>[2x]GPLGSMHNVLIVGASRGIGLGLADAFLQRGAQVFAVARRPQGSPGLQALAERAGERLQAVTGDLNQHDCA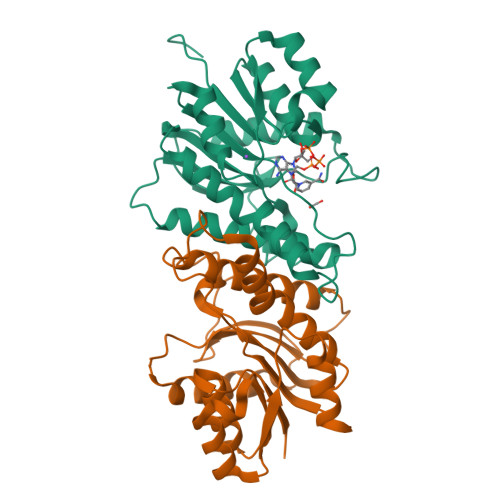ERIGEMLGERRIDRLIVNAGIYGPQQQDVAEIDAEQTAQLFLTNAIAPLRLARALSGRVSRGGVVAFMSSQMASLALGLSATMPLYGASKAALNSLVRSWEGEFEELPFSLLLLHPGWVRTEMGGDSAPLSVEESAAGLVAAVEDAAGVNACRFVDYRNQPLPW1,4-DIDEOXY-1,4-IMINO-L-ARABINITOL 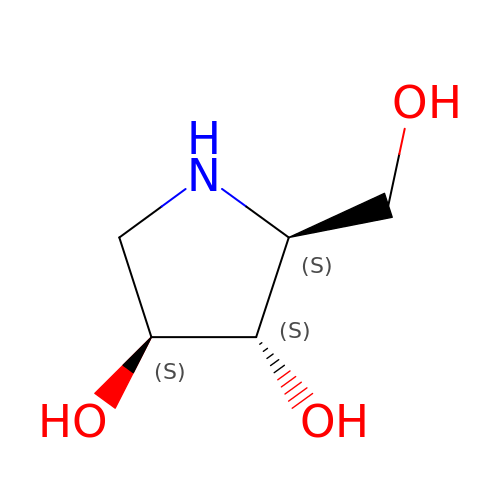| C5 H11 N O3 | OQEBIHBLFRADNM-YUPRTTJUSA-N5-(3-azanylpropylamino)pentyl-$l^{3}-oxidanyl-bis(oxidanyl)boron | C8 H22 B N2 O3 | 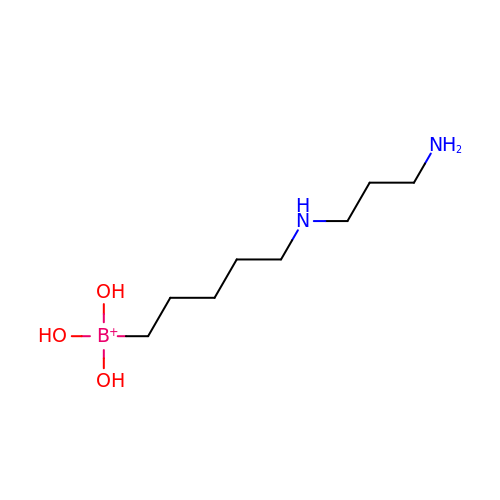RWZPDLKEHZSJIC-UHFFFAOYSA-N Nuclear respiratory factor 1 (NRF1) regulates the expression of genes that are vital for mitochondrial biogenesis, respiration, and various other cellular processes. NRF1 was initially identified as a transcription activator of cytochrome c by binding to the cytochrome c promoter as a homodimer. Subsequently, a consensus sequence GCGCNTGCGC (N represents any nucleotide) was identified as the DNA binding motif of NRF1 (6), which has also been detected in the promoters of many other nuclear genes relevant to mitochondrial biogenesis and respiration, such as the promoters of reductase (ubiquinone-binding protein) complex (6), cytochrome oxidase assembly factor COX17 (7), myocyte enhancer factor 2A (MEF2A), and ferridoxin reductase (FDXR). Our structural, mutagenesis and luciferase reporter assay results revealed that, although the NRF1 DBD alone is capable of recognizing the TGCGC DNA motif, the cooperativity between DD and DBD is essential for the binding of the intact GCGCATGCGC sequence and the transcriptional activity of NRF1.

To investigate this, we expressed the NRF1 DBD fragment (aa 177–284) alone and assessed its binding affinity to the 14bp dsDNA that we used for crystallization. Our ITC data showed that the NRF1 DBD binds to this dsDNA with a Kd of ∼1.4 μM, albeit ∼5-fold weaker than the NRF1 dimer. Subsequently, we successfully determined one complex structure of the NRF1 DBD bound to a 16bp dsDNA with a sequence GGTGCGCATGCGCACC. This 16bp dsDNA exhibits a comparable binding affinity to the NRF1 DBD as the 14bp dsDNA. In the NRF1 DBD–16pb dsDNA complex, only one NRF1 DBD molecule and a single DNA strand are observed in an asymmetric unit (ASU), and the complementary DNA strand from another ASU binds to another NRF1 molecule. In addition to the interactions between the NRF1 molecule and the DNA in one ASU, its symmetry-related NRF1 molecule from the other ASU also contributes to the electrostatic and base interactions with the DNA duplex, which results in two NRF1 DBDs bound to a DNA duplex. Structural analysis shows that the residues R206, N242 and R244 from each DBD molecule interact specifically with one TGCGC motif, similar to what is observed in the NRF1 dimer-dsDNA complex structure. Mutations of any of these residues of DBD led to a significant reduction or complete loss of binding between NRF1 DBD and the 16bp dsDNA. In the NRF1 DBD-dsDNA complex, the two DBD molecules bind separately to the two TGCGC motifs of the GGTGCGCATGCGCACC DNA, approaching the DNA duplex from nearly the same side with a tail-to-tail-like orientation. However, in the NRF1 dimer-dsDNA complex, the DD restricts the orientation of the DBD, enabling the two DBDs to bind to the intact GCGCATGCGC motif from nearly the opposite sides of the DNA duplex in a head-to-head orientation.

> GAPQEVNSELPPLTIDGIPVSVDKMTQAQLRAFIPEMLKYSTGRGKPGWGKESCKPIWWPEDIPWANVRSDVRTEEQKQRVSWTQALRTIVKNCYKQHGREDLLYAFED>EDPPACGSIVPRREWRALASECRERLTRPVRYVVVSHTAGSHCDTPASCAQQAQNVQSYHVRNLGWCDVGYNFLIGEDGLVYEGRGWNIKGAHAGPTWNPISIGISFMGNYMNRVPPPRALRAAQNLLACGVALGALRSNYEVKGHRDVQPTLSPGDRLYEIIQTWSHYRA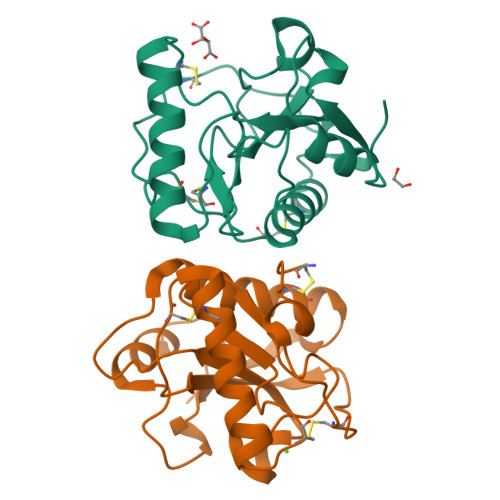[4x]> MGLENIRDAVRKFLTGSTPYEKAVDEFIKDLQKSLISSDVNVKLVFSLTAKIKERLNKEKPPSVLERKEWFISIVYDELSKLFGGDKEPNVNPTKLPFIIMLVGVQGSGKTTTAGKLAYFYKKRGYKVGLVAADVYRPAAYDQLLQLGNQIGVQVYGEPNNQNPIEIAKKGVDIFVKNKMDIIIVDTAGRHGYGEETKLLEEMKEMYDVLKPDDVILVIDASIGQKAYDLASRFHQASPIGSVIITKMDGTAKGGGALSAVVATGATIKFIGTGEKIDELETFNAKRFVSRILGMGDIESILEKVKGLEEYDKIQKKMEDVMEGKGKLTLRDVYAQIIALRKMGPLSKVLQHIPGLGIMLPTPSEDQLKIGEEKIRRWLA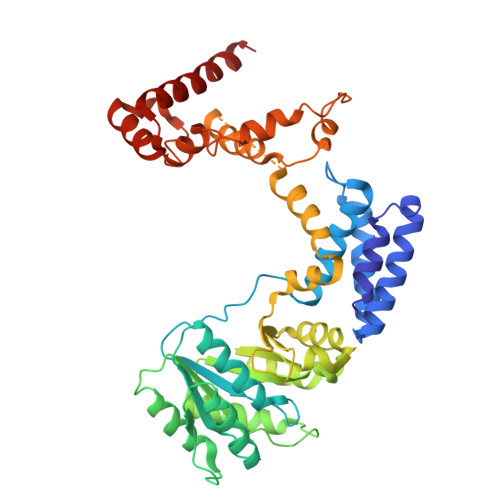ALNSMTYKELENPNIIDKSRMRRIAEGSGLEVEEVRELLEWYNNMNRLLKMVK> DCPPDWSSYEGHCYRFFKEWMHWDDAEEFCTEQQTGAHLVSFQSKEEADFVRSLTSEMLKGDVVWIGLSDVWNKCRFEWTDGMEFDYDDYYLIAEYECVASKPT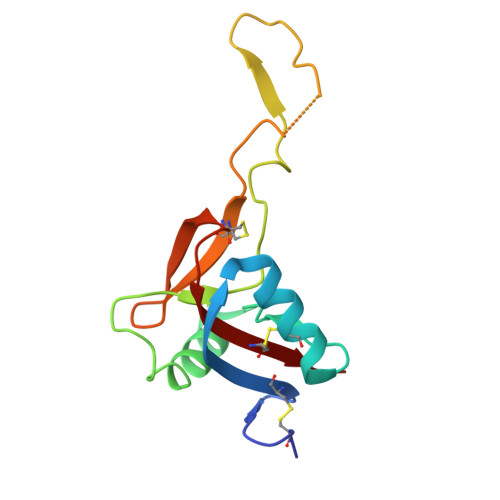NNKWWIIPCTRFKNFVCEFQA>[2x]MAGKSSLFKVILLGDGGVGKSSLMNRYVTNKFDTQLFHTIGVEFLNKDLEVDGHFVTMQIWDTAGQERFRSLRTPFYRGSDCCLLTFSVDDSQSFQNLSNWKKEFIYYADVKEPES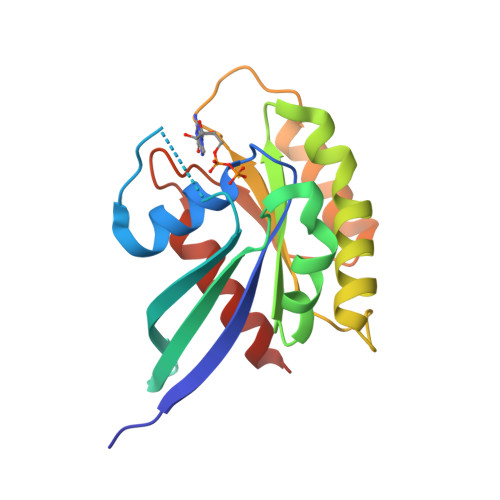FPFVILGNKIDISERQVSTEEAQAWCRDNGDYPYFETSAKDATNVAAAFEEAVRRVLATED> MVVTFLQDLEVLQDALLNNLQKLSAISRRKESGESKHDNKDSFAAIANEHNDEEEEIEFEDLVNIIESKVSDFESVLKCSIVEMTYKYPELKLQWEKSPRYDQCDKLHIVKLDKQMNEDIYAQLVEELDFVLQFVDWFYCYRLKVKEILRQHHKRDLAWND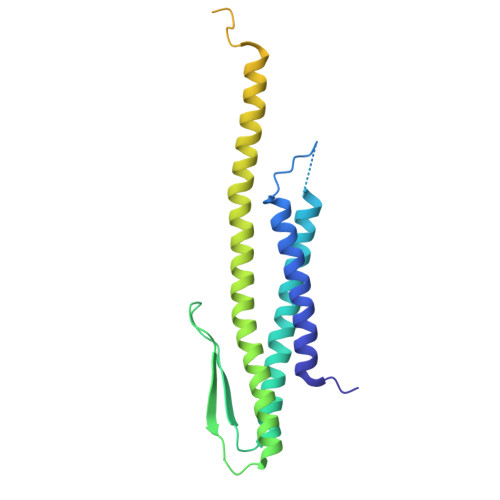EKRDRAIKFHAVDYDKLHQGTSSSSSLTSTSMEKASTREKLLSKTKQLTNNLVRGNQILQSGILQSDLNLDELRAQTNSLTQIDDKYTQFETVFKKTADLVKVLENASHQEKRD>SAKDERAREILRGFKLNWMNLRDAETGKILWQGTEDLSVPGVEHEARVPKKILKCKAVSRELNFSSTEQMEKFRLEQKVYFKGQCLEEWFFEFGFVIPNSTNTWQSLIEAAPESQMMPASVLTGNVIIETKFFDDD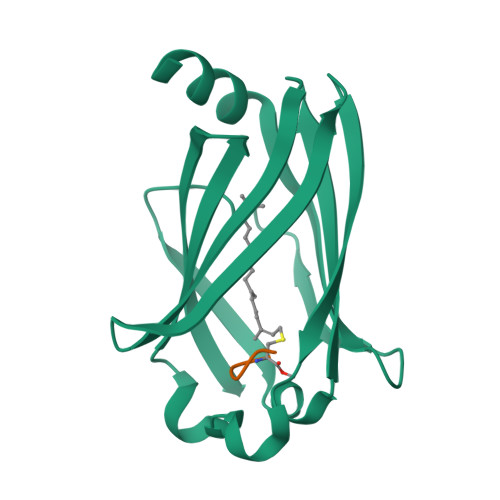LLVSTSRVRLFYV[2x];>KSKTC[2x]>[6x]ADVFHLGLTKAMLDGATLAIVPGDPERVKRIAELMDNATFLASHREYTSYLAYADGKPVVICSTGIGGPSTSIAVEELAQLGVNTFLRVGSTGAIQPHVNVGDVIVTQASVRLDGASLHFAPMEFPAVANF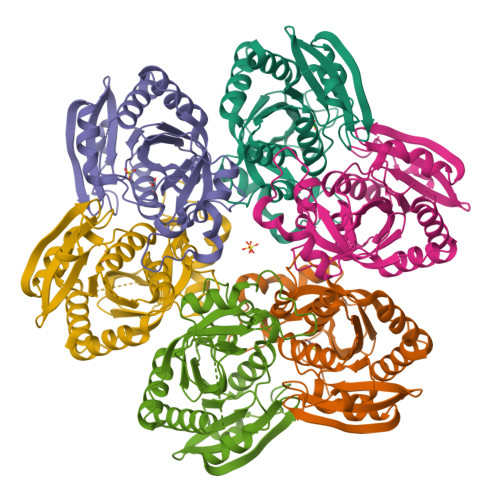ECTTAMVAACRDAGVEPHIGVTASSDTFYPGQERYDTVTGRVTRRFAGSMKEWQDMGVLNYEMESATLFTMCATQGWRAACVAGVIVNRTQQEIPDEATMKKTEVSAVSIVVAAAKKLLA ethyl (9S)-9-[5-(1H-benzimidazol-2-ylsulfanyl)furan-2-yl]-8-hydroxy-5,6,7,9-tetrahydro-2H-pyrrolo[3,4-b]quinoline-3-carboxylate 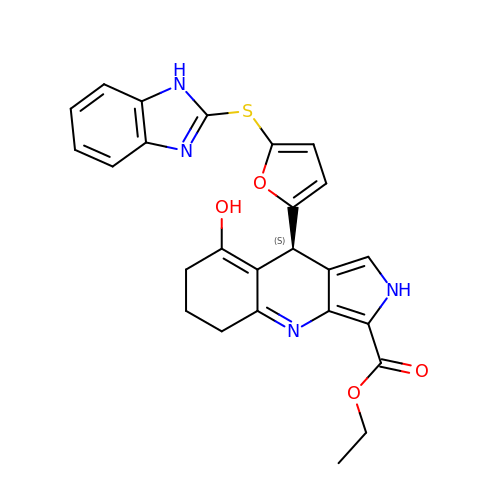| C25 H22 N4 O4 S | POXQKNUAFHJFKI-HXUWFJFHSA-N> MALSGHVLIDPARLPRDTGPELMWAPSLRNSLRVSPEALELAEREAERARSERWDRCAQVLKNRLLRVELDGIMRDHLARAEEIRQDLDAVVAFSDGLESMQVRSPSTGGRSAPAPPSPSPAQPFTRLTGNAQYAVSISPTDPPLMVAGSLAQTLLGNLYGNINQWVPSFGPWYRTMSANAMQRR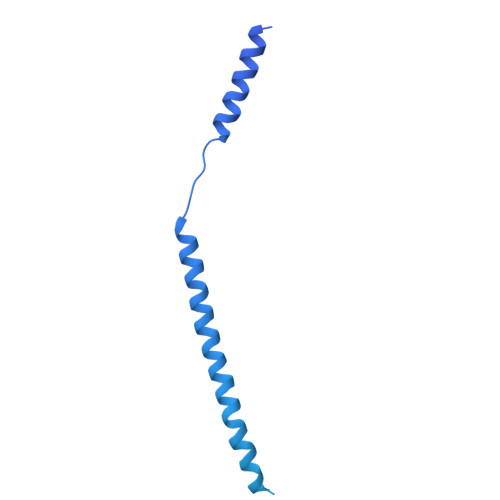VFPKQLRGNLNFTNSVSLKLMTEVVAVLEGTTQDFFSDVRHLPDLQAALILSVAYLLLQGGSSHQQRPLPASREELLELGPESLEKIIADLKAKSPGGNFMILTSGNKEARQSIAPLNRQAAYPPGTFADNKIYNLFVGAGLLPTTAALNVPGAAGRDRDLVYRIANQIFGEDVPPFSSHQWNLRVGLAALEALMLVYTLCETANLAEAATRRLHLSSLLPQAMQRRKPAMASAGMPGAYPVQTLFRHGELFRFIWAHYVRPTVAADPQASISSLFPGLVLLALELKLMDGQAPSHYAINLTGQKFDTLFEIINQKLLFHDPAAMLAARTQLRLAFEDGVGVALGRPSPMLAAREILERQFSASDDYDRLYFLTLGYLASPVAPS3-(3-chlorophenoxy)-1-[(piperidin-4-yl)methyl]-1H-pyrazolo[3,4-d]pyrimidin-4-amine 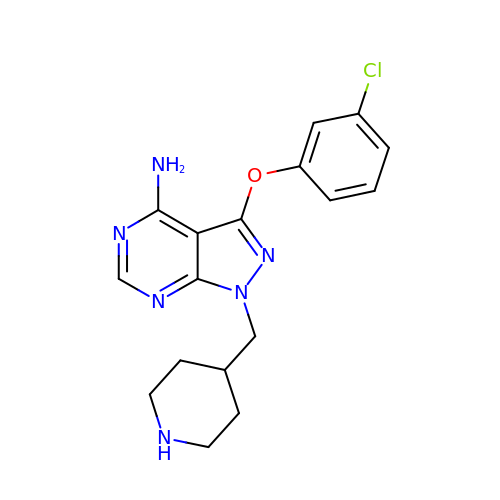| C17 H19 Cl N6 O | HYRFAZNYCCTVKT-UHFFFAOYSA-N> 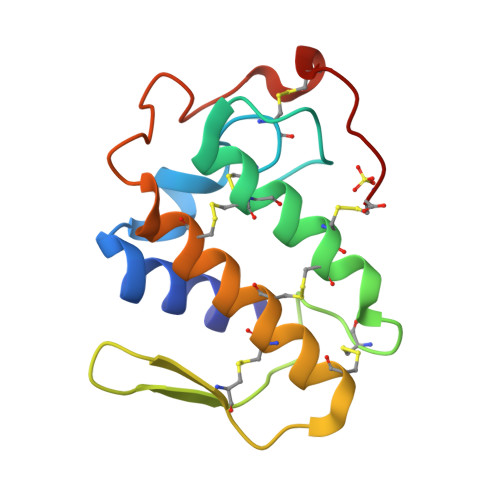NLYQLWKMILQETGKNAAPSYGFYGCNCGVGSRGKPKDATDRCCFVHKCCYKALTDCSPKTDSYSYSWKDKTIVCGKNNPCLKQECECDKAVAICLRDNLDTYNKNYKIYPKPLCKKADDC>MGSEDNIKETFFISHGTPMMAIDDSKPSKKFLESWREKIFSKKPKAILVISAHWETDQPSVNVVDINDTIYDFRGFPARLYQFKYSAPGSPELANRIQDLLAGSGFKSVNTDKKRGLDHGAWVPLMLMYPEADIPVCQLSVQSHLDGTHHYKLGQALAPLKDEGVLIIGSGSATHPSNGTPPCSDGVAPWAAAFDSWLETALTNGSYEEVNKYETKAPNWKLAHPWPEHFYPLHVAMGAAGENSKAELIHNSWDGGIMSYGSYKFTSTLEHHHHHH[2x]

The biosynthesis of betalains involves the enzymatic action of 4,5-DOPA-dioxygenase, which catalyzes the key ring-opening reaction of DOPA to produce betalamic acid, a crucial intermediate in the pathway. DOPA-4,5-dioxygenase (DOD) is an enzyme that catalyzes extradiol aromatic ring cleavage. BvDOD belongs to the extradiol dioxygenase superfamily and catalyzes the conversion of L-DOPA into betalamic acid. In this study, the properties of BvDOD were characterized, and the first crystal structure of this plant-type DOPA-dioxygenase was determined.

Crystals were successfully obtained by screening and optimizing the conditions for purified BvDOD and diffracted to 3.08 Å. The crystal structure of BvDOD, which included 263 amino acid residues (Asn6–Thr268) and one Fe atom, was ultimately refined to an Rwork of 16.70% and an Rfree of 22.00%. The crystal structure of BvDOD conformed to the P3121 space group and accommodated two molecules per asymmetric unit. Superimposition of the Cα coordinates from the two molecules revealed a root-mean-square deviation of 0.186 Å, which highlighted the high degree of structural consistency between the two forms. The enzyme displayed a single-domain structure with a mixed eight-strand β-sheet surrounded by 10 α-helices. The α/β-fold, comprising a central β-sheet flanked by two clusters of α-helices, was a hallmark of its structural architecture. A crucial feature of BvDOD was the presence of an interior pocket containing a mix of hydrophobic and hydrophilic regions accessible from the exterior. This pocket, approximately 20 Å deep and 585 Å3 in volume, was strategically positioned to facilitate substrate binding and catalysis. In the substrate-free form, the Fe ion within the active site was coordinated by the oxygen atoms of three water molecules and the Nε2 atoms of three histidine residues (His15, His53, and His229). These residues were strategically located within loops that connected β1-α1, β2-β3, and α9-α10, respectively, playing a crucial role in maintaining the active site’s structural integrity.>GRGYEIPARLRTLHNLVIQYASQGRYEVAVPLCKQALEDLEKTSGHDHPDVATMLNILALVYRDQNKYKDAAHLLNDALAIREKTLGKDHPAVAATLNNLAVLYGKRGKYKEAEPLCKRALEIREKVLGKFHPDVAKQLSNLALLCQNQGKAEEVEYYYRRALEIYATRLGPDDPNVAKTKNNLASCYLKQGKYQDAETLYKEILTRAHEKEFGSVNGENKPIWMHAEEREESKDKRRDSAPYGEYGSWYKACKVDSPTVNTTLRSLGALYRRQGKLEAAHTLEDCASRSR[2x];>GPGGRMGKEVGNLLLENSQLLETKNALNVVKNDLIAKVDQLSGEQEVLKGELEAAKQAKVKLENRIKELEEELKR[2x]

Kinesin-1 transports numerous cellular cargoes along microtubules. The kinesin-1 light chain (KLC) mediates cargo binding and regulates kinesin-1 motility. KLC comprises an N-terminal heptad repeat region that oligomerizes with the KHC stalk, an acidic linker region, and a tetratricopeptide repeat (TPR) domain containing six TPRs (TPR1-6) (Gauger and Goldstein, 1993, Verhey et al., 1998, Wong and Rice, 2010, Zhu et al., 2012). The KLC TPR domain (KLCTPR) is unusual in binding to multiple ligands using distinct sites (Hammond et al., 2008, Zhu et al., 2012).

To investigate the molecular mechanisms of kinesin-1 recruitment and activation by JIP3/4, and how this is regulated by ARF6, we determined the crystal structure of the murine KLC2 TPR domain (KLC2TPR) in complex with the murine JIP3LZ to a resolution of 3.2 Å. The crystallographic asymmetric unit contains a single copy of the complex, which comprises two copies of KLC2TPR bound to one copy of the JIP3LZ dimer, which adopts a parallel coiled-coil conformation. The KLCTPR binds JIP3LZ end-on, via TPR1. This was unanticipated, since TPR domain ligands usually bind to the concave inner surface. The KLC2 TPR1 α helices pack flat against the side of the JIP3LZ, lying across the JIP3LZ helices at a ∼90° angle, and oriented with helix 1B proximal to the JIP3LZ N terminus. This buries 571 Å2 of surface area on each KLC2TPR. The KLC2TPR binding site spans heptad repeats 2–5 (residues 433–435, 437–442, 444–446, and 450) of the JIP3LZ. The JIP3LZ hydrophobic patch is recognized by a number of hydrophobic side chains that line the inside of KLC2 TPR1 (Leu201, Leu204, Tyr208, Val216, and Leu220). Around the edge of the hydrophobic core of the KLC2TPR:JIP3LZ interface, the side chains of KLC2 residues Thr200 and Tyr208 (TPR1 helix A), and Gln223 and Asp227 (helix B), hydrogen bond to the side chains of JIP3 residues Asp450, Asp444, Lys435, and Asn439. Comparison with the crystal structure of the ARF6:JIP4LZ complex shows that the KLC and ARF6 binding sites on the JIP3/4LZ overlap, consistent with KLC and ARF6 competing directly for binding (Montagnac et al., 2009).>QHHHHHHAAKFSVEAGAGFYGGFGGQLAVVAEDLAPGLPLGVRLGVGFATSDALDDGYDLGGGTTWGDVKEAGKFSEWGQNVTLSLDVLYKPSGLGLPVEVAPYFGVRYNFFSGGYTDPEDNLTIKAQTISSNQLGLGLGVRAAYPLMPNLSLVGDLGVDYYFQACFTRVEEDDSGNKSQSSVCPGDSGYE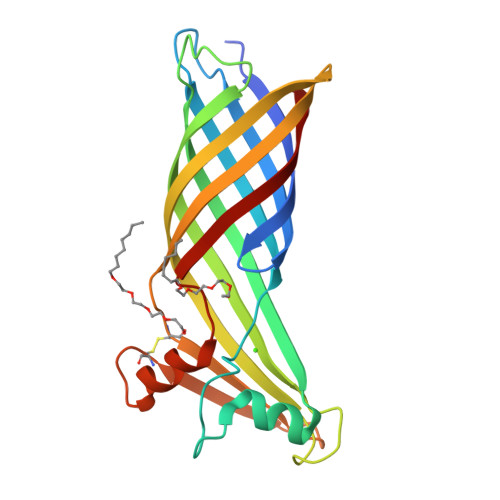DVNKFVTQPEWVLKLRLGAAYRF[3x]>GSESLLYGYFL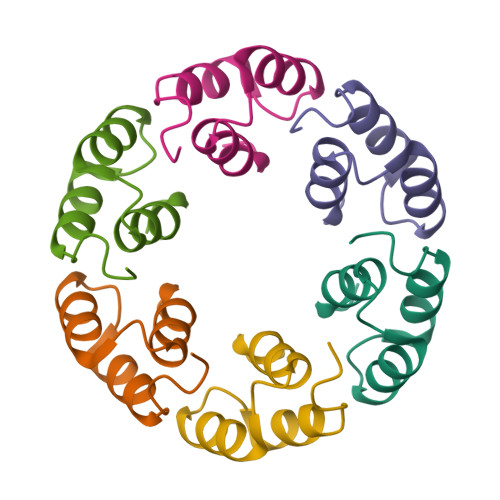DSWLDGTASEELLRVAVNAGDLTQEEADKIMSYPWGAWND[6x]> GAQKRHITQQHLRRTAEAEEQWKLQAKEIEAGRKQSFLSFLEERGLVNSVVGQRDALDKLITRKRVGFYAGVDPTAPSLHIGHMLPFMILGWAYVHGLKAVFLIGGSTAKIGDPTGRLEGRPLMDGATRRANIANIHLQLKRLGFSFEKYGRKHGFEWEWAWRRALENNNTWWNKQSLKEVMEVLGTSLRLGPMLGRDYVKSRLASGEGMSIAEFCYPIMQGWDFWYLFQRKVQVQVGGSDQYGNILFGMDAIKGILKANPESEWAPKKDEDPDLANPYGITTPLLTTASGEKIGKSAG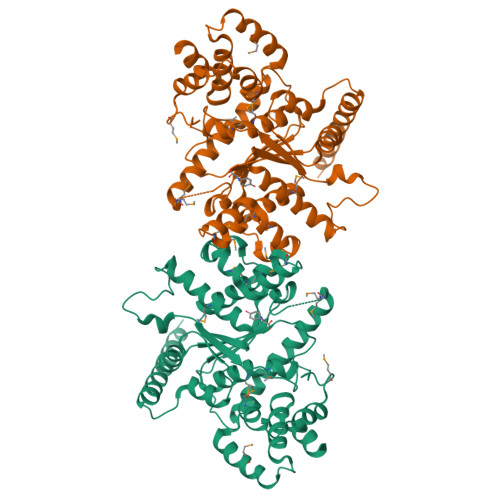NAVWLDKDMTSCYDLYQYFVRVADSDVERYLKMFTFVPTPAIKELMEEHAKDPSKRVAQHKLAREFVELIHGSLSAEQAAKDHRT5-fluoro-N-methyl-2-(7H-pyrrolo[2,3-d]pyrimidin-5-yl)pyrimidin-4-amine 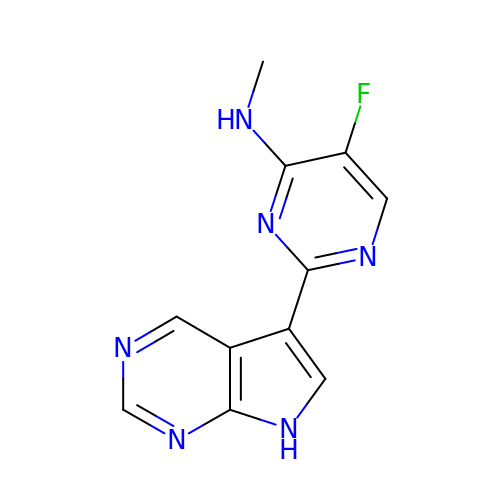| C11 H9 F N6 | VCAWVIOIVGOEIB-UHFFFAOYSA-N> PATPTASSSSST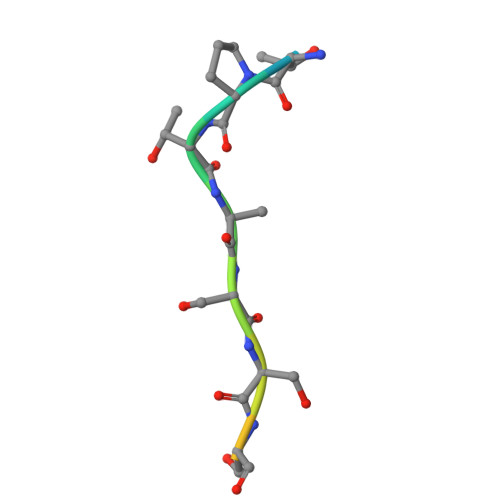TPT2-[(2-{[1-(N,N-dimethylglycyl)-5-methoxy-1H-indol-6-yl]amino}-7H-pyrrolo[2,3-d]pyrimidin-4-yl)amino]-6-fluoro-N-methylbenzamide 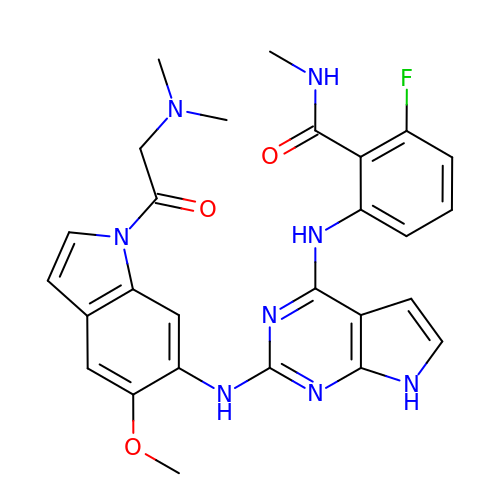| C27 H27 F N8 O3 | DESOLSKAHZZIGK-UHFFFAOYSA-N>[5x]MFVPWQLGTITRHRDELQKLLAASLLPEHPEESLGNPIMTQIHQSLQPSSPCRVCQLLFSLVRDSSTPMGFFEDYACLCFFCLYAPHCWTSTMAAAADLCEIMHLHFPEEEATYGLFGPGRLMGIDLQLHFFVQKCFKTTAAEKILGISNLQFLKSEFIRGMLTGTITCNFCFKTSWPRTDKEEATGPTPCCQITDTTTAPASGIPELARATFCGASRPTKPSLLPALID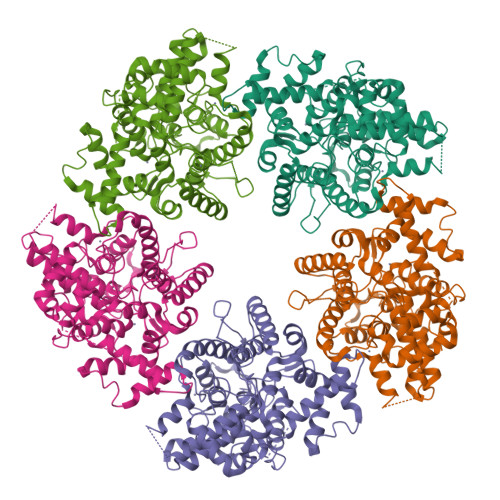IWSTSSELLDEPRPRLIASDMSELKSVVASHDPFFSPPLQADTSQGPCLMHPTLGLRYKNGTASVCLLCECLAAHPEAPKALQTLQCEVMGHIENNVKLVDRIAFVLDNPFAMPYVSDPLLRELIRGCTPQEIHKHLFCDPLCALNAKVVSEDVLFRLPREQEYKKLRASAAAGQLLDANTLFDCEVVQTLVFLFKGLQNARVGKTTSLDIIRELTAQLKRHRLDLAHPSQTSHLYA> TICADGTSVANGACCKLIPVVKDLTENLFEGECGDAAHGALRLVFHDAIAISPTLGGGGADGSIAVFNATELTFHANTGIDDVLDAVGPFLLKHSDVMTPGDFIQLAGAVSLTQCNGAPRVKFVMGRPPPKAAAPNLLVPEPFDSVATILQRFGELGFTKEETVAVIGGSHSVAGADDIVPNEQGIPFDQTPSIFDTQIFVDVQLRGTMIPGNGTTEGEVETAVPGTVRLQSDHLLARDASTSCIWQSFVNQQSKMAQVFGEAIFKMSLLGQTQSKLIDCSEVIPRAIPFSHGPATLPPGQTLKDIEQACAASPFPTLSTQPGPVTSVPAIP

Manganese peroxidases (MnPs) are, together with lignin peroxidases and versatile peroxidases, key elements of the enzymatic machineries secreted by white-rot fungi to degrade lignin, thus providing access to cellulose and hemicellulose in plant cell walls. The primary mechanism involves the MnP oxidation of Mn2+ to Mn3+ and the subsequent formation of chelates with fungal dicarboxylic acids. The molecular structures of Ape-MnP1 and Cst-MnP1, which share 50% amino acid sequence identity, are characteristic of ligninolytic peroxidases.

As a consequence, using Ape-MnP1 and Cst-MnP1 as representatives of the subfamilies they belong to, we renamed both subfamilies as MnP-DDQ, with a manganese oxidation site made up of Asp/Asp/Gln; and MnP-ED, with a manganese oxidation site formed by Glu/Asp. It was surprising to find that the MnP-DDQ subfamily differs from previously characterized MnPs in two of the three residues involved in Mn2+ coordination, with Asp35 and Gln333 in Ape-MnP1 occupying the position of two glutamate residues in short and long/extra-long MnPs. Comparison of the crystal structures of Mn-free Ape-MnP1 and Mn-bound Ape-MnP1 shows that the Asp35 side chain occupies different positions. In addition, Gln333 located at the C-terminal end does not even appear in the Mn-free Ape-MnP1 structure due to the predicted mobility of this region in the absence of the cation. The different orientation of the Asp35 side chain in the structures of substrate-bound and substrate-free Ape-MnP1, and the absence of Gln333 in the crystal structure of the Mn-free enzyme, confirm the mobility of these residues, a behavior that has also been demonstrated for the two glutamates of the Mn2+ oxidation site in previously characterized MnPs. The movements of these two residues witness the dynamic nature of the Mn2+ oxidation site in Ape-MnP1, a dynamic that is different from that reported for MnP of P. chrysosporium and VP of Pleurotus eryngii, since the C-terminal tails of the latter are not involved in Mn2+ coordination. The kinetic constants of Ape-MnP1-Q333P confirmed that Gln333 participates in Mn2+ binding (a 172-fold decrease in Mn2+ affinity was observed for the mutated variant) but not in its oxidation (kcat was hardly impaired). Accordingly, based on these results and the structural studies described above, we propose that the position of the Asp35 and Gln333 side chains in Mn-free Ape-MnP1 corresponds to an “open-gate” conformation of the active site, necessary for cation uptake. The subsequent reorientation of the side chains of these two residues pointing toward the Mn2+ ion in Mn-bound Ape-MnP1 corresponds to the “closed-gate” conformation, in which the enzyme oxidizes the cation in direct contact with the internal heme propionate after being activated by H2O2. The substrate-free Ape-MnP1 model differs from the substrate-bound enzyme in the number of solvent molecules (207 in the Mn2+-free enzyme).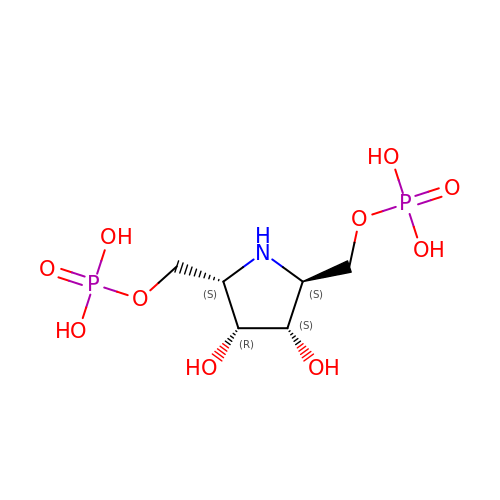[(2S,3R,4S,5S)-3,4-dihydroxypyrrolidine-2,5-diyl]bis(methylene) bis[dihydrogen (phosphate)] | C6 H15 N O10 P2 | JDMJAXIARMVOFV-OMMKOOBNSA-N> MERLAPAKVNLGLSVRFRREDGYHELHTLFAPFSLADRLVVEPVSSGLHFQGPYGRENLAYRAASLYLEAAGQPGGVRILLEKRIPEGAGLGGGSSDAAQVLLALQALYPAEVDLFALARTLGADVPFFLLGRGAEARGVGERLKPLALPPVPAVVFFPGLRVPTPLVYRAVRPEDFGPDLPVEAILEALARGEEPPYWNSLEGPAFRLFPELKEVR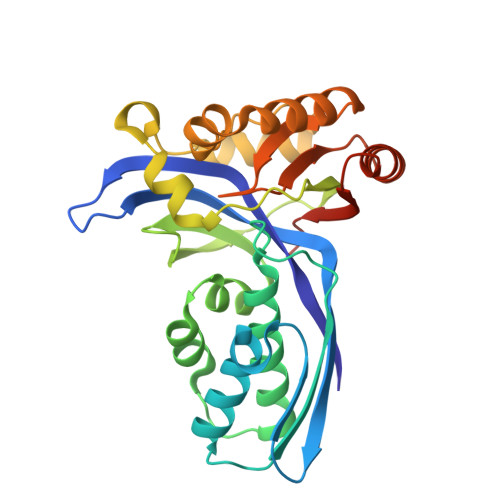GRMRALGLRGVLMSGSGSAFFGLAEGPDHARRAAEALRAWGRAWAGTLGGGDAGSGPA2,6-DICARBOXYNAPHTHALENE | C12 H8 O4 | 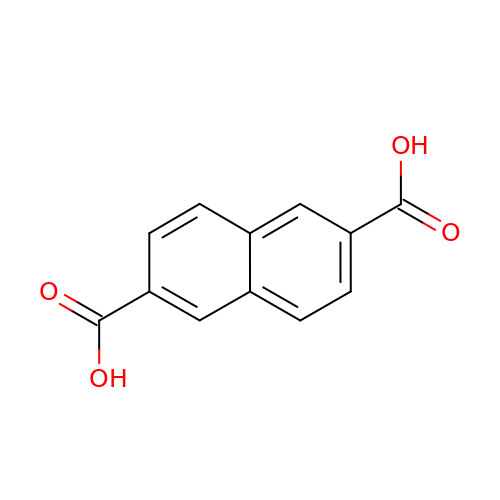RXOHFPCZGPKIRD-UHFFFAOYSA-N> MAQIVDVYGNPIRTQQLREPQTSRLAGLAKEFAQHPAKGLTPAKLARILVEAEQGNLQAQAELFMDMEERDAHLFAEMSKRKRAILGLDWAVEPPRNASAAEKADADYLHELLLDLEGLEDLLLDALDGIGHGYSCIELEWALQGREWMPLAFHHRPQSWFQLNPEDQNELRLRDNSPAGEALQPFGWIIHRPRARSGYVARSGLFRVLAWPYLFRHYATSDLAEMLEIYGLPIRLGK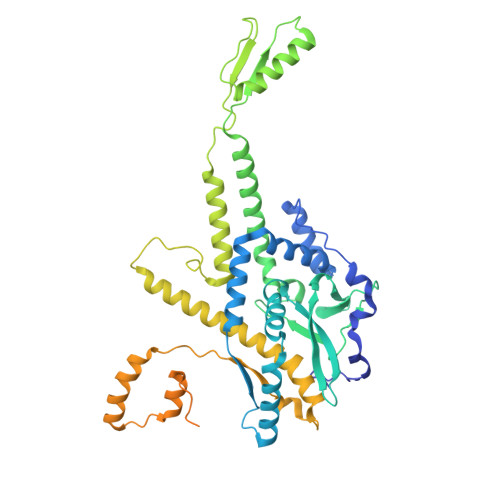YPPGTADEEKATLLRAVTGLGHAAAGIIPETMAIDFQQAAQGSSDPFLAMMRQSEDAISKAVLGGTLTSTTSQSGGGAFALGQVHNEVRHDLLASDARQLAATLSRDLLWPLLVLNRPGSPDVRRAPRLVFDLREQADITSMAQSIPALVNVGLEIPSAWVYDKLGIPQPAKNEPVLRSAAQPAILSRQHGQRVAALATIVGPRYGDQQALDKALASLPAKDMQDQVNDLLAPLLEAVNRGDSETELLGALAEAFPDMDDSALTDALHRLLFAADTWGRLHGNLDRID> MSVFPGLCGDVATTNYRVFLGTLPNLAVEERFLRQVQPVFPWYASRKHVKEQASEFLEIDLASCDPELLLRYTHVYYVRRQLYDELVDRQLTLMETGKAAKVADSALLTCLAQVNAAITPRLQYELHLLQQAKKACRVPRRRELNPDAALEAHDYLCMMRVVEEDVGGIPDAEMQARAYLPREVLEAKVKELAAMIFGDGGSATKGTGAALERKEQKLLQRMIPADYNKVGAVEKLRPVDVTALYRFTGERVCGRPADKPFARALWGHVFRKVGSHPLYLQRASLYWARHSGLDPQSATSAMPADLATAVCVQQALFPALKYRCQYLYTSPDIARQQWRTGHVVPLLRLFPLLGAPAAEDLAAQLVVEGEWAKLGIEADTNLLHDTVLRQ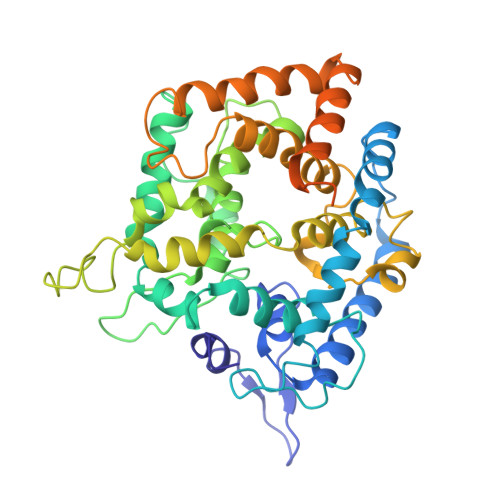LKDMVEQVSALYESDAGAVLKRVEDGAKVLCPSLSERESLTMRGAPEDTSREVSAAAAARVANAAPA COENZYME 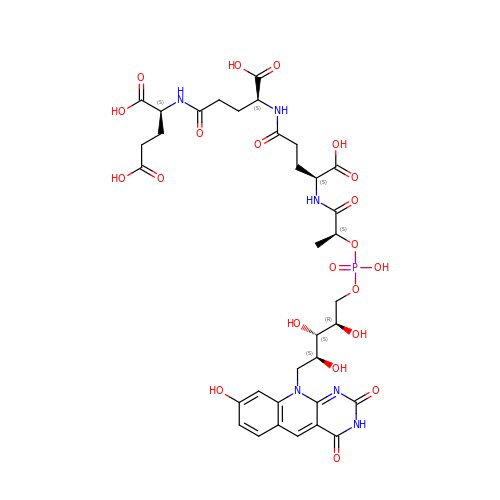F420-3 | C34 H43 N6 O21 P | YHDAXCLOUDHUAA-LROHGRLLSA-N>MAHAGRTGYDNREIVMKYIHYKLSQRGYEWDAGDDVEENRTEAPEGTESEVVH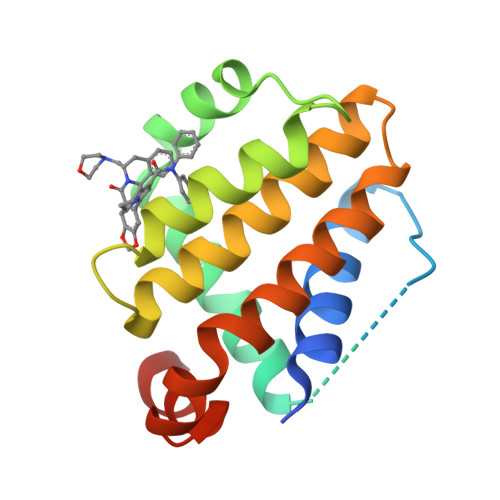LTLRQAVDDFSRRYRRDFAEMSSQLHLTPFTARGRFATVVEELFRDGVNWGRIVAFFEFGGVMCVESVNREMSPLVDNIALWMTEYLNRHLHTWIQDNGGWDAFVELYGPSMR[2x]>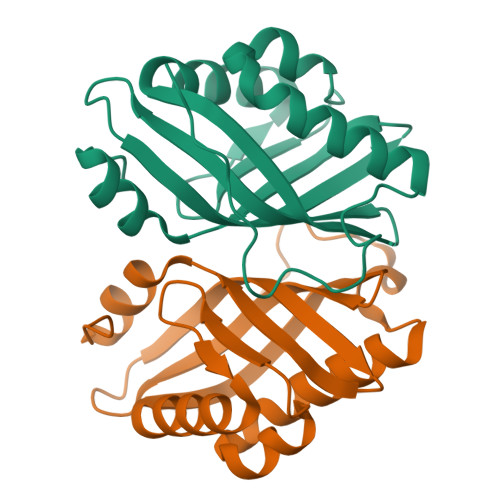[4x]MHHHHHHTSKIEQPRWASKDSAAGAASTPDEKIVLEFMDALTSNDAAKLIEYFAEDTMYQNMPLPPAYGRDAVEQTLAGFFTVFSIDAVETFHIGSSNGLVYTERVDVVRALPTGKSYNVSVLGVFQLTEGKITGWRDYFDLREVEEAVDLPVRG>[2x]STVYNINLGIGWASSGVEYAQAYRAQILRRIQQPAKFIFMDMILADNIQHLTENIGFLDEEIIWLYNYFTDIKIAPTTVTLDQVLAQVAGQPERSEKEGKIVRYFYPQDDQFITCYLRQEDQDFVEHVEYVSRGRLIRKDYFSYVRYASEYFAPHNDAATLYQRRFYHEDGSVAYDMLIEDGQEKLYRFPDRIFYSKAELVRYFLQCLQLQADDVVILDRETGIGQVVFEESQKAKLGVVVHAEHFSENASSDDYILWNNFYDYQFTNADKVDFFIVATEAQKRILEQQFQHYSDKQPQIATIPVGSLDQLTYPKEPRKPYSMITASRLATEKHIDWLVAATVQAHAQLPELT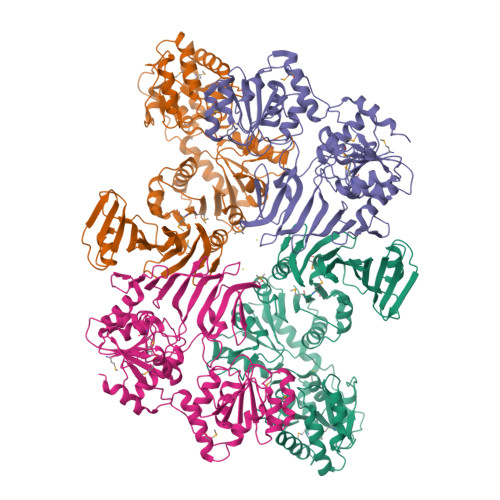LDIYGKGSEEDKLRRRIEEAGAQDYIRLKGHADLSQIYAGYELYLTASTSEGFGLTLMEAVGSGLPLIGFDVRYGNQTFIDDGKNGYLLPVSSNHVEDQIIAAFVEKIIALFSQGRQQEMSQHSYQVAENYLTSRVEAAWTQLLKEVRDD;>MIQLFDYYNQETQDLHDSLLAAGYACPTIVIEANGFLPDDMISPYTYFLGDEEGVDHPLFFNQVPVPPFWEITGDHQVARVSDMGEERARIHYASQARGRLVKQVDWLDKKGQLRLSERYNKQGRCFAKTAYKSGQEAFNTTYYSTDGQERIVENHVTGDIILTLDQEPLRIFKSRVDFIRFFLERLDLDLDHILFNSLAYSFLVSHSLTGRAGQDILFWQEPLYDELPGNMQLILDNSQLRTQTIVIPDLATYEKAMSLAAADQQQKFLHLGYHYDFKRDNYLRKDALILTHSDQIEGLDTLVQSLPQLVFRIAALTEMSPKLLSMLSYKNVVLYQNASLKQIEQLYLESDIYLDINHGGQVLQAVRKAFENNLLILGFEQTLHDRHYIAQQHIFDSSQPAQLASILEEALCGVEQMRSALQAQGRHANDVPVSLYQETLQSLLGG[2x]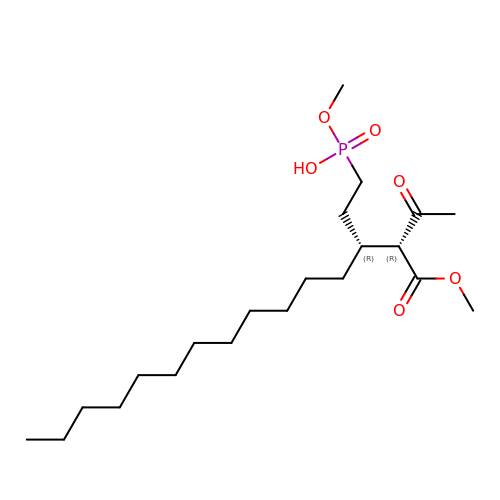methoxy-[(3~{R})-3-[(2~{R})-1-methoxy-1,3-bis(oxidanylidene)butan-2-yl]pentadecyl]phosphinic acid | C21 H41 O6 P | VBHWHUMRWJDMHN-UXHICEINSA-N> GIIL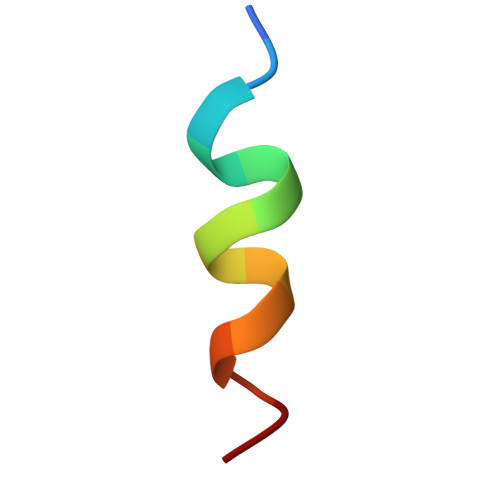VLLIWGTVLL> GDRVADVIESSIGDSVSRALTHALPAPTGQNTQVSSHRLDTGKVPALQAAEIGASSNASDESMIETRCVLNSHSTAETTLDSFFSRAGLVGEIDLPLKGTTNPNGYANWDIDITGYAQMRRKVELFTYMRFDAEFTFVACTPTGEVVPQLLQYMFVPP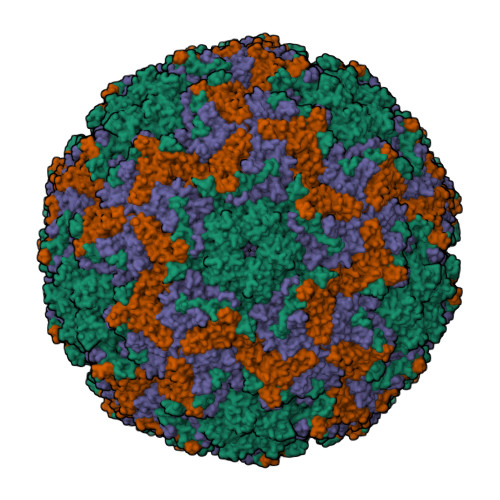GAPKPDSRESLAWQTATNPSVFVKLSDPPAQVSVPFMSPASAYQWFYDGYPTFGEHKQEKDLEYGAMPNNMMGTFSVRTVGTSKSKYPLVVRIYMRMKHVRAWIPRPMRNQNYLFKANPNYAGNSIKPTGASRTAITTL;> SPSAEACGYSDRVAQLTIGNSTITTQEAANIIVGYGEWPSYCSDSDATAVDKPTRPDVSVNRFYTLDTKLWEKSSKGWYWKFPDVLTETGVFGQNAQFHYLYRSGFCIHVQCNASKFHQGALLVAVLPEYVIGTVAGGTGTEDTHPPYKQTQPGADGFELQHPYVLDAGIPISQLTVCPHQWINLRTNNCATIIVPYINALPFDSALNHCNFGLLVVPISPLDYDQGATPVIPITITLAPMCSEFAGLRQAVTQ;> GFPTELKPGTNQFLTTDDGVSAPILPNFHPTPCIHIPGEVRNLLELCQVETILEVNNVPTNATSLMERLRFPVSAQAGKGELCAVFRADPGRNGPWQSTLLGQLCGYYTQWSGSLEVTFMFTGSFMATGKMLIAYTPPGGPLPKDRATAMLGTHVIWDFGLQSSVTLVIPWISNTHYRAHARDGVFDYYTTGLVSIWYQTNYVVPIGAPNTAYIIALAAAQKNFTMKLCKDASDILQTGTIQ;> MGSQVSTQRSGSHENSNSATEGSTINYTTINYYKDSYAATAGKQSLKQDPDKFANPVKDIFTEMAAPLK>MHHHHHHMETGPEDPSSMPEESSPRRTPQSIPYQDLPHLVNADGQYLFCRYWKPTGTPKALIFVSHGAGEHSGRYEELARMLMGLDLLVFAHDHVGHGQSEGERMVVSD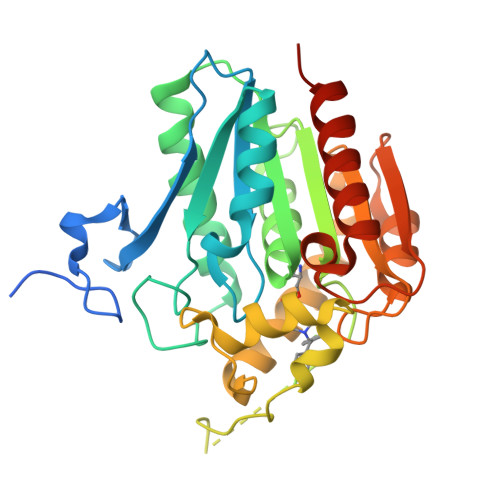FHVFVRDVLQHVDSMQKDYPGLPVFLLGHSMGGAIAILTAAERPGHFAGMVLISPLVLANPESATTFKVLAAKVLNLVLPNLSLGPIDSSVLSRNKTEVDIYNSDPLICRAGLKVCFGIQLLNAVSRVERALPKLTVPFLLLQGSADRLCDSKGAYLLMELAKSQDKTLKIYEGAYHVLHKELPEVTNSVFHEINMWVSQRTATAGTASPP[2x]>[2x]GSHMTATTGPPPKLCLVCSDE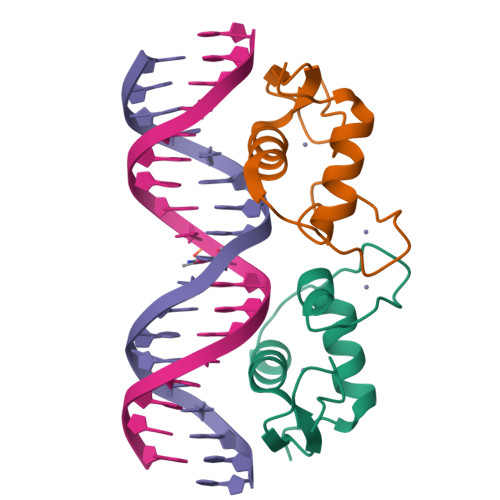ASGCHYGVLTCGSCKVFFKRAVEGQHNYLCAGRNDCIIDKIRRKNCPACRYRKCLQAGMNLEARKTKKKIKGI> APQQINDIVHRTITPLIEQQKIPGMAVAVIYQGKPYYFTWGYADIAKKQPVTQQTLFELGSVSKTFTGVLGGDAIARGEIKLSDPTTKYWPELTAKQWNGITLLHLATYTAGGLPLQVPDEVKSSSDLLRFYQNWQPAWAPGTQRLYAGSSIGLFGALAVKPSGLSFEQAMQTRVFQPLKLNHTWINVPPAEEKNYAWGYREGKAVHVSP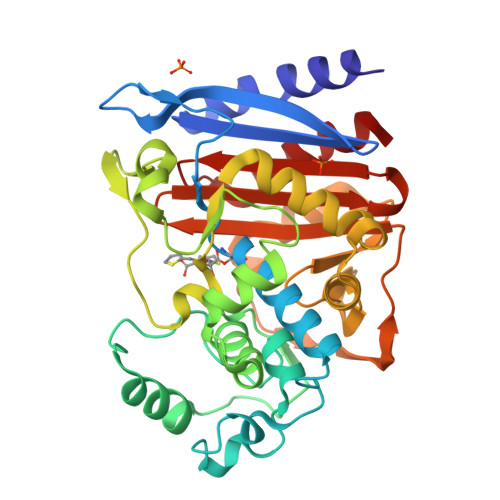GALDAEAYGVKSTIEDMARWVQSNLKPLDINEKTLQQGIQLAQSRYWQTGDMYQGLGWEMLDWPVNPDSIINGSDNKIALAARPVKAITPPTPAVRASWVHKTGATGGFGSYVAFIPEKELGIVMLANKNYPNPARVDAAWQILNALQ> MRPSGTAGAALLALLAALCPASRALEEKKVCQGTSNK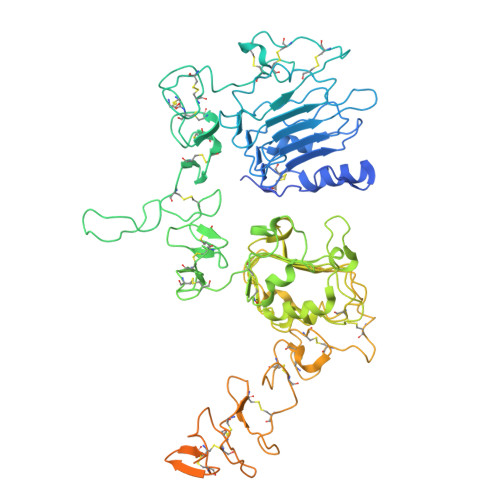LTQLGTFEDHFLSLQRMFNNCEVVLGNLEITYVQRNYDLSFLKTIQEVAGYVLIALNTVERIPLENLQIIRGNMYYENSYALAVLSNYDANKTGLKELPMRNLQEILHGAVRFSNNPALCNVESIQWRDIVSSDFLSNMSMDFQNHLGSCQKCDPSCPNGSCWGAGEENCQKLTKIICAQQCSGRCRGKSPSDCCHNQCAAGCTGPRESDCLVCRKFRDEATCKDTCPPLMLYNPTTYQMDVNPEGKYSFGATCVKKCPRNYVVTDHGSCVRACGADSYEMEEDGVRKCKKCEGPCRKVCNGIGIGEFKDSLSINATNIKHFKNCTSISGDLHILPVAFRGDSFTHTPPLDPQELDILKTVKEITGFLLIQAWPENRTDLHAFENLEIIRGRTKQHGQFSLAVVSLNITSLGLRSLKEISDGDVIISGNKNLCYANTINWKKLFGTSGQKTKIISNRGENSCKATGQVCHALCSPEGCWGPEPRDCVSCRNVSRGRECVDKCNLLEGEPREFVENSECIQCHPECLPQAMNITCTGRGPDNCIQCAHYIDGPHCVKTCPAGVMGENNTLVWKYADAGHVCHLCHPNCTYGCTGPGLEGCPTNGPKIPSIATGMVGALLLLLVVALGIGLFMRRRHIVRKRTLRRLLGGSENLYFQGGGSAAQLKKKLQALKKKNAQLKWKLQALKKKLAQSNSLEVLFQ> FMVSLPRMVYPQPK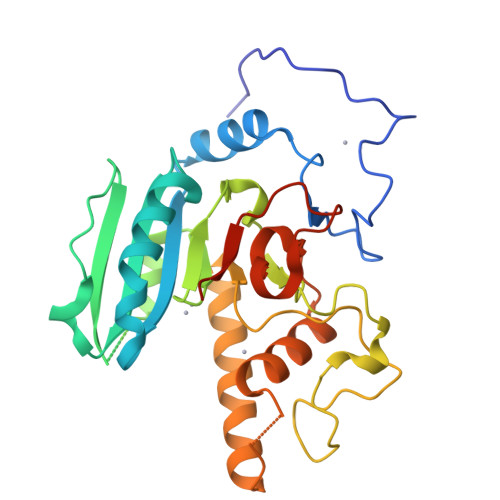VLTPCRKDVLVVTPWLAPIVWEGTFNIDILNEQFRLQNTTIGLTVFAIKKYVAFLKLFLETAEKHFMVGHRVHYYVFTDQPAAVPRVTLGTGRQLSVLEVGAYKRWQDVSMRRMEMISDFCERRFLSEVDYLVCVDVDMEFRDHVGVEILTPLFGTLHPSFYGSSREAFTYERRPQSQAYIPKDEGDFYYMGAFFGGSVQEVQRLTRACHQAMMVDQANGIEAVWHDASHLNKYLLRHKPTKVLSPEYLWDQQLLGWPAVLRKLRFTAVPKNHQAVRNPE>[2x]GMATETLTKSDAITQSLRAAVDRNFNDQVAFLQRMVQFRSVRGEEAPQQEWLAQQFADRGYKVDTFSLADVDIASHPKAAPMDTIDPAGSMQVVATADSDGKGRSLILQGHIDVVPEGPVDLWSDPPYEAKVRDGWMIGRGAQDMKGGVSAMIFALDAIRTAGYAPDARVHVQTVTEEESTG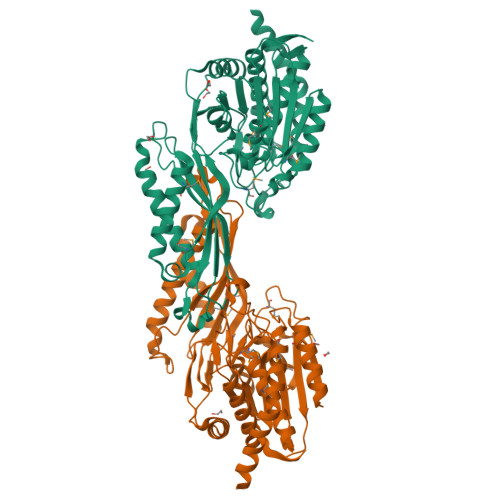NGALSTLMRGYRADACLIPEPTGHTLTRAQVGAVWFRLRVRGTPVHVAYSETGTSAILSAMHLIRAFEEYTKELNAQAVRDPWFGQVKNPIKFNVGIIKGGDWASSTAAWCELDCRLGLLTGDTPQEAMRGIEKCLADAQATDSFLSENPAELVWSGFQADPAVCEPGGVAEDVLTAAHKAAFNAPLDARLSTAVNDTRYYSVDYGIPALCYGPYGQGPHAFDERIDLESLRKTTLSIALFVAEWCGLRKL>[2x]MTISLNHTIVPAHNKEASAQFFAQIFGLNVSSVGHFAAVRVNDT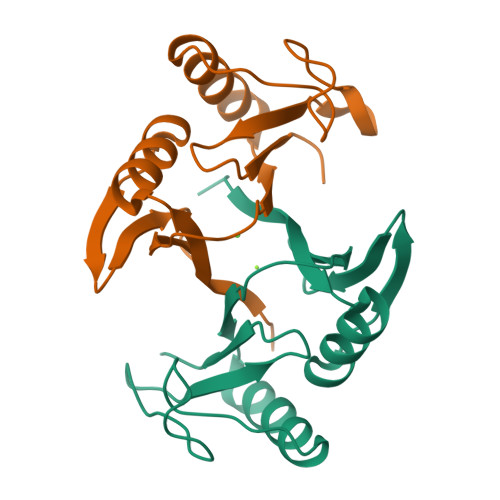LTLDFDDRETFESHHYAFHVSDEEFDTIFARIKQAGLEYSSDPMHHNKGEINHRKGGRGFYFYDPNGHNLELLTLS> L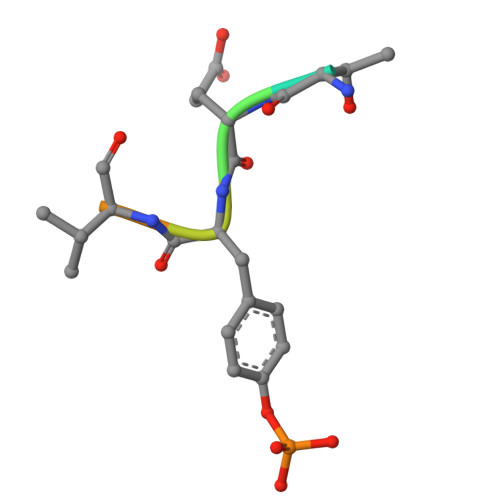TEYVATR>[3x]LTAKHRPSVVWLHNAECTGCTEAAIRTIKPYIDALILDTISLDYQETIMAAAGEAAEAALHQALEGKDGYYLVVEGGLPTIDGGQWGMVAGHPMIETTKKAAAKAKGIICIGTCSAYGGVQKAKPNPSQAKGVSEALGVKTINIPGCPPNPINFVGAVVHVLTKGIPDLDENGRPKLFYGELVHDNCPRLPHFEASEFA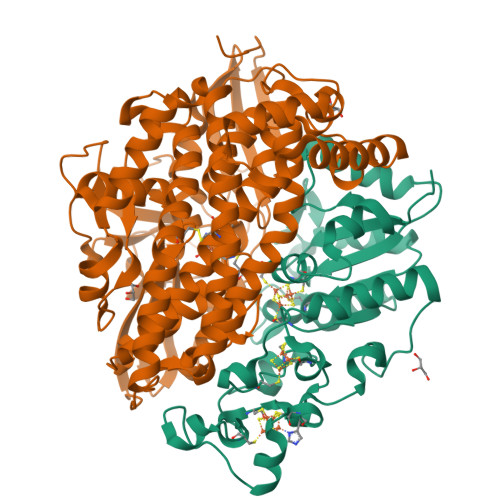PSFDSEEAKKGFCLYELGCKGPVTYNNCPKVLFNQVNWPVQAGHPCLGCSEPDFWDTMTPFYEQG;>[3x]MAESKPTPQSTFTGPIVVDPITRIEGHLRIMVEVENGKVKDAWSSSQLFRGLEIILKGRDPRDAQHFTQRACGMCTYVHALASSRCVDDAVKVSIPANARMMRNLVMASQYLHDHLVHFYHLHALDWVDVTAALKADPNKAAKLAASIAPARPGNSAKALKAVQDKLKAFVESGQLGIFTNAYFLGGHKAYYLPPEVDLIATAHYLEALHMQVKAASAMAILGGKNPHTQFTVVGGCSNYQGLTKDPLANYLALSKEVCQFVNECYIPDLLAVAGFYKDWGGIGGTSNYLAFGEFATDDSSPEKHLATSQFPSGVITGRDLGKVDNVDLGAIYEDVKYSWYAPGGDGKHPYDGVTDPKYTKLDDKDHYSWMKAPRYKGKAMEVGPLARTFIAYAKGQPDFKKVVDMVLGKLSVPATALHSTLGRTAARGIETAIVCANMEKWIKEMADSGAKDNTLCAKWEMPEESKGVGLADAPRGALSHWIRIKGKKIDNFQLVVPSTWNLGPRGAQGDKSPVEEALIGTPIADPKRPVEILRTVHAFDPCIACGVH>MMEQVCDVFDIYAICACCKVESKNEGKKNEVFNNYTFRGLGNKGVLPWKCISLDMKYFRAVTTYVNESKYEKLKYKRCKYLNKETVDNVNDMPNSKKLQNVVVMGRTNWESIPKKFKPLSNRINVILSRTLKKEDFDEDVYIINKVEDLIVLLGKLNYYKCFILGGSVVYQEFLEKKLIKKIYFTRINSTYECDVFFPEINENEYQIISVSDVYTSNNTTLDFIIYKKTNNKMLNEQNCIKGEEKNNDMPLKNDDKDTCHMKKLTEFYKNVDKYKINYENDDDDEEEDDFVYFNFNKEKEEKNKNSIHPNDFQIYNSLKYKYHPEYQYLNIIYDIMMNGNKQSDRTGVGVLSKFGYIMKFDLSQYFPLLTTKKLFLRGIIEELLWFIRGETNGNTLLNKNVRIWEANGTREFLDNRKLFHREVNDLGPIYGFQWRHFGAEYTNMYDNYENKGVDQLKNIINLIKNDPTSRRILLCAWNVKDLDQMALPPCHILCQFYVFDGKLSCIMYQRSCDLGLGVPFNIASYSIFTHMIAQVC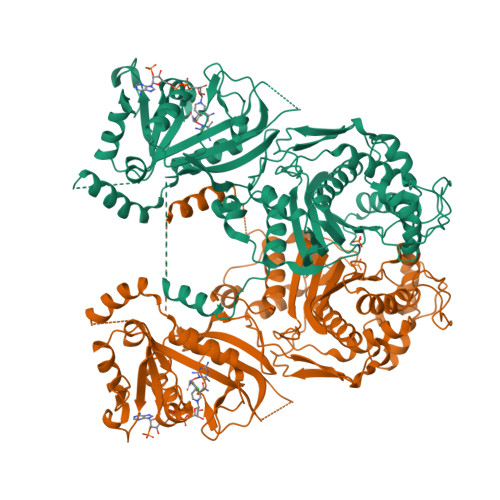NLQPAQFIHVLGNAHVYNNHIDSLKIQLNRIPYPFPTLKLNPDIKNIEDFTISDFTIQNYVHHEKISMDMAA[2x]> SEDSRPAAHFHLSSRRRHQGSMGYHGDMYIGNDNERNSYQGHFQTRDGVLTVTNTGLYYVYAQICYNNSHDQNGFIVFQGDTPFLQCLNTVPTNMPHKVHTCHTSGLIHLERNERIHLKDIHNDRNAVLREGNNRSYFGI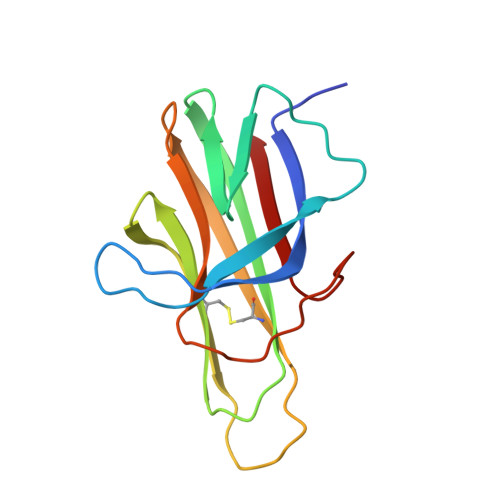FKV>QNVGTQAAEEPLNLPISVCTAPGNCQTEADAVVLDSNWRWAHTTTGYTNCYTGNLWDTTLCPTPETCTTNCAIDGVPLADWSGTYGGSVTGNKFNLKFVTVGPYSTNIGARTFLLDSTKTRYRMFQLLNREFTYDVDVSSLDCGLNGALYFVSMDADGGAAKYPTNKGGAKYGTGYCDAQCPHDVKWINGLANSKDWTPIPGDANSGKGYYGNCCAELDIWEANKQSQAFTTHPCTPNDQTRCEGVVCGDNDSGDRYNGMCDKDGCDFASYRMNDHTFYGPGSTFKLDSTKPFTVVSQFITTDGTDNGDFKEFRRFYVQNGVRIENSKVNFPGITAYDSITDEMCAATKGLFGDLDDHKNKGGMKQMGEAMRKGMALVMSIWDDHDVNMLWLDSNYPPTGNPSTPGVARGPCPTTSGVPSEVEVTQANAVVSFGNIKFGPIGSTV[2x]

During macromolecular X-ray crystallography experiments, protein crystals held at 100 K have been widely reported to exhibit reproducible bond scission events at doses on the order of several MGy. OH-cleavage from tyrosine residues is regularly cited as amongst the most available damage pathways in protein crystals at 100 K, despite a lack of widespread reports of this phenomenon in protein crystal radiation damage studies. A systematic investigation performed on a range of protein crystal damage series deposited in the Protein Data Bank has established that Tyr –OH electron density loss is not generally a dominant damage pathway in protein crystals at 100 K. Full Tyr aromatic ring displacement is here proposed to account for instances of observable Tyr –OH electron density loss, with the original myrosinase data shown to be consistent with such a damage model. To better characterize the reproducibility of Tyr –OH group electron density loss in irradiated protein crystals, we have performed a systematic investigation on a wide range of structures at 100 K. A subset of previously conducted MX radiation damage investigations have included deposition of readily accessible coordinate and structure factor information in the Protein Data Bank (PDB), providing an ideal database of protein damage series.

Regardless of the feasibility of a radiation-induced Tyr –OH damage event within crystalline protein at 100 K, Tyr –OH density loss is in general significantly lower than for Glu and Asp carboxyl­ates for doses >1 MGy, at which de­carboxyl­ation events were reported. Prominent Tyr –OH density loss did not appear to be a widespread feature of general protein structures, a finding that is consistent with the high energetic barrier for Tyr phenolic C—O bond scission.~{N}-[2-[[6-chloranyl-3-[4-methoxy-3-[[(2~{R})-1-oxidanylbutan-2-yl]sulfamoyl]phenyl]-2-methyl-imidazo[1,2-b]pyridazin-8-yl]amino]ethyl]ethanamide 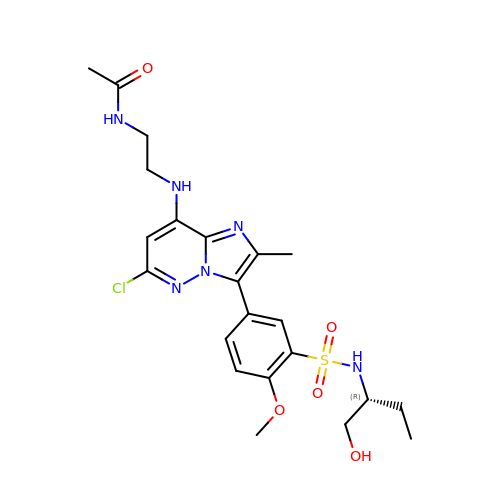| C22 H29 Cl N6 O5 S | FWLVCDHZPISLAA-MRXNPFEDSA-N> PTVEEV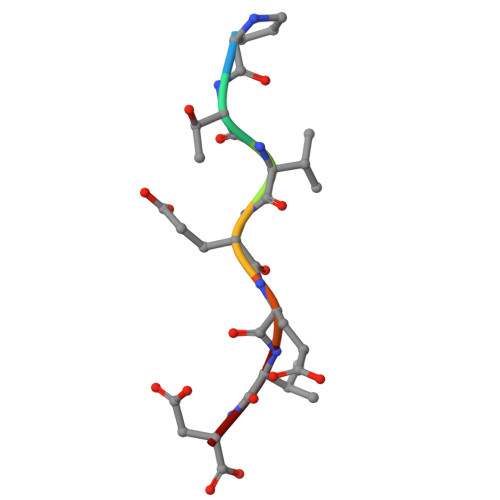D> HESKQSIMQRI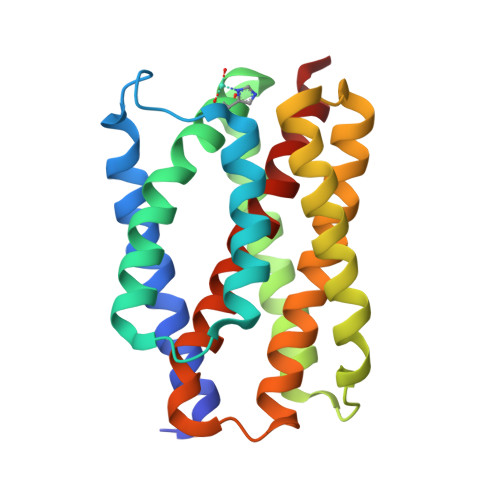LTVFVFTLLIATVGLFIGQFVPVALMLPLSILEVAMIILAFWMRRRKAVGYAFVYTFAFVSGITLFPIVSHYASIAGAYVVLEAFGSTFVIFAVLGTIGAKMKKDLSFLWSFLLVAVLALAVVGIFNIFSPLNSAAMMAYSVIGTIVFSLYILYDLNQIKHRHITEDLIPVMALSLYLDFINLFINLLRFFGILSSDD>[2x]ACDYTCGSNC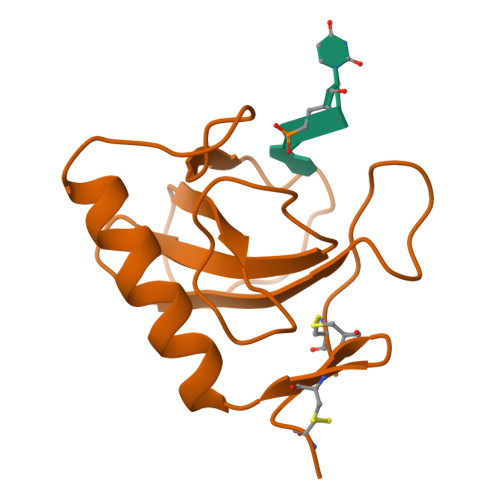YSSSDVSTAQAAGYQLHEDGETVGSNSYPHKYNNYEGFDFSVSSPYYEWPILSSGDVYSGGSPGADRVVFNENNQLAGVITHTGASGNNFVECT>[2x]MIVQLGKASVTWTRADLEAKLAGHA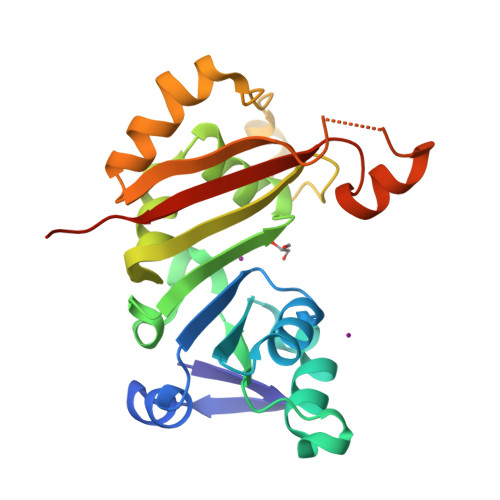RVLIDVGTGDGRFVYRSAGAHPDTYCIGVDPAGERMREVSWRASRKPARGGRPNALFVVASVQALPEELAGLAHTLTLNFPWASLLSALVLPEAPVLEALRRLVRPGGELIALLNQSVFDDRPYAARLGLPELSDAWLDDALRPAYRAAGFEIRTSEIVDGEVPHQTSWGQHLTLASGRRTRLLTAEAIGGSASAAPG> MVIATDDLEVACPK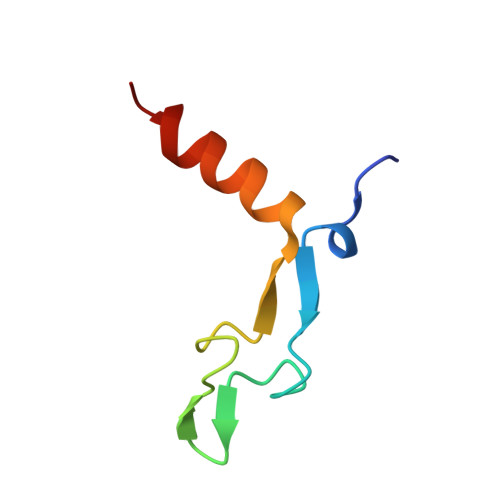CERAGEIEGTPCPACSGKGVILTAQGYTLLDFIQKHLNK NA, which is a sialidase, catalyzes hydrolysis of terminally linked sialic acid and functions as the receptor-destroying element of influenza A and B viruses. Additionally, influenza A NA is further classified into two groups: group 1 (N1, N4, N5 and N8) and group 2 (N2, N3, N6, N7 and N9), based upon primary sequence. Group 1 NAs contain a 150-cavity (formed by amino acids 147–151 of the 150-loop) in their active site, whereas group 2 NAs lack this cavity. NA inhibition assays were carried out and complex crystal structures were solved for laninamivir, laninamivir octanoate, zanamivir and oseltamivir in order to elucidate the structural basis of their inhibition.

N5 on the other hand contains Val149 with no 147–150 salt bridge and displays a 150-cavity like all other structure-known NAs with Val149 and no 147–150 salt bridge. To determine the structural basis of the inhibition of laninamivir relative to zanamivir, we solved the very first complex structures of laninamivir with p57N2, p09N1 and N5 at resolutions of 1.8 Å, 1.8 Å and 1.6 Å, respectively; and the complex structures of zanamivir with p57N2, p09N1 and N5 at 1.9 Å, 1.9 Å and 1.6 Å, respectively. The typical group 1 N5 contains a 150-cavity in its uncomplexed structure and inhibition of N5 by laninamivir and zanamivir was better than inhibition of p09N1 and p57N2, which contain no 150-cavity in their uncomplexed structures. Unlike p09N1 and p57N2, N5 contains Tyr347, which forms an additional hydrogen bond with the carboxylate of each inhibitor. The additional hydrogen bond between Tyr347 and the inhibitor carboxylate is also a key factor in explaining the higher N5 inhibition relative to p09N1 and p57N2. However, like the closed 150-loop, this residue also makes the active site cavity smaller and in this way may also limit access of inhibitors to the N5 active site. In the open state of the 150-loop, when the 150-cavity is formed, Asp151 shifts over 1.5 Å (the Asp151 Cγ is shifted over 2 Å in N5) away from the ligand binding site, which should facilitate entry of inhibitors like zanamivir and laninamivir. The typical group 1 N5 contains a 150-cavity in its uncomplexed structure and inhibition of N5 by both laninamivir and zanamivir was the highest. Therefore, we provide structural and functional evidence that the open 150-loop of a typical group 1 NA may facilitate the entry of the 4-guanidino group of zanamivir and laninamivir into the NA active site, relative to the closed 150-loop of group 2 NAs. Laninamivir was in a similar range with zanamivir for N5, p09N1 and p57N2 with IC50 values of 0.90 nM, 1.83 nM and 3.12 nM, respectively.

>PEFLNNTEPLCNVSGFAIVSKDNGIRIGSRGHVFVIREPFVACGPTECRTFFLTQGALLNDKHSNNTVKDRSPYRALMSVPLGSSPNAYQAKFESVAWSATACHDGKKWLAVGISGADDDAYAVIHYGGMPTDVVRSWRKQILRTQESSCVCMNGNCYWVMTDGPANSQASYKIFKSHEGMVTNEREVSFQGGHIEECSCYPNLGKVECVCRDNWNGMNRPILIFDEDLDYEVGYLCAGIPTDTPRVQDSSFTGSCTNAVGGSGTNNYGVKGFGFRQGNSVWAGRTVSISSRSGFEILLIEDGWIRTSKTIVKKVEVLNNKNWSGYSGAFTIPITMTSKQCLVPCFWLEMIRGKPEERTSIWTSSSSTVFCGVSSEVPGWSWDDGAILPFDIDKM[2x]>[2x]MKNRIDPELRAMLDMFPPLNLDDVQATRKAMEEAAQLTELPVDEEVVVSNRMVPGPEDNPYVRVRIYEPKEKIEKLPGLLWIHGGGYVLGAPEGDDLLCQRFVKEANCVVVSVDYRLAPEHPYPAPLEDCYAALQWFAKKVDELGVDASRIGVGGQSAGGGLTAALALLARDRKGPELCFQMPLYPMIDDKNNSPSSLEITGNLIWNHDLNEKGWSMYLDGKNGTDDVPVHAAPARATDLTNLPYTYTCVGQLDPFRDETLDYVKRLCQAGVDVEFHLYPGAYHGFETLNPAAAVSQRALAEYVGAVKHVLNREKVVERK

Here we determine the structure of a novel hormone sensitive lipase (HSL) family IV cold active esterase (EstN7) isolated from Bacillus cohnii strain N1 to understand the basis of cold adaptation. EstN7 is a member of the HSL (or IV) family with a α/β hydrolase fold and consists of a central eight stranded β-sheet surrounded by nine helices. Unlike many esterases isolated from psychrophilic organisms that still have optimal enzyme activity at greater than 20°C, EstN7 is truly cold active with an optimal temperature of 5–10°C with a dramatic drop-off in activity above 20°C. We have previously shown that EstN7 retained function in the presence of up to 30% of various organic solvents, which makes it potentially useful in a variety of applications, such as fine chemical synthesis and pharmaceutical industries. Esterases are particularly useful as they catalyse the hydrolysis of a wide variety of esters into their constituent alcohol and acid.

EstN7 was observed as a dimer in the unit cell, which was confirmed in solution by size exclusion chromatography. The two β-sheets are connected across the dimer interface via an antiparallel arrangement of strand 8 from each subunit to form effectively a single continuous sheet, with residues in the C-terminal helix and helix 8 also contributing. The active site lies at the bottom of the cleft formed by the cap region and comprised Ser157, Asp254 and His284. In both subunits, S157 adopts two distinct hydroxymethyl rotamers with approximately 115° between the two. Electron density that equates to ethylene glycol was also observed in the active site of both subunits, with an additional ethylene glycol found in subunit B. Analysis of EstN7 solvent accessible surface area (SASA) shows that the second helix-loop (residues 23–40) is not tightly associated with the catalytic domain as is the case in related structures but forms a bridge-like structure that reveals additional potential tunnels to the active site not present in the closely related mesophilic and thermophilic esterases. The bridge structure is anchored by M31 and L40 through hydrophobic interactions; the connecting residues do not form any additional interactions with the rest of the protein. The calculated volume of the active site using CASTp is 1026 and 1148 Å3 for the A and B subunit, respectively. Surface electrostatics were calculated using APBS (Adaptive Poisson–Boltzmann Solver) and revealed the surface of EstN7 is largely negative with a few basic patches. Thus, EstN7's cold adaptation mechanism is likely to include dealing with change in water entropy and allowing improved access for substrate to the active site.>[4x]MCGNTMSVPLLTDAATVSGAERETAAVIFLHGLGDTGHSWADALSTIRLPHVKYICPHAPRIPVTLNMKMVMPSWFDLMGLSPDAPEDEAGIKK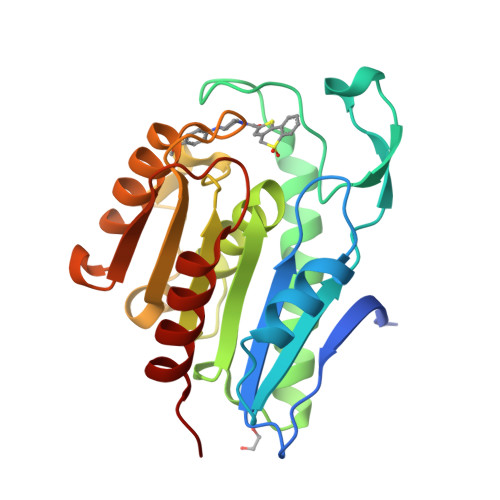AAENIKALIEHEMKNGIPANRIVLGGFSQGGALSLYTALTCPHPLAGIVALSCWLPLHRAFPQAANGSAKDLAILQCHGELDPMVPVRFGALTAEKLRSVVTPARVQFKTYPGVMHSSCPQEMAAVKEFLEKLLPPV>[3x]MLEANVYDNFNPNYYNISDFSMPNGKKEKRGLPIPKARCQVINYELWETGYLYTSSATLTVSVEVGDIVQILFPEVVPIEEALGKKKKLNLDMVYLVTDVDESNKATLKNYFWAMIESLDVPNAITKTTNFAIIDYLIDPNKNNLMSYGYFFNSSIFAGKATINRKAETSSAHDVAKRIFSKVQFQPTTTIQHAPSETDPRNLLFINFASRNWNRKRITTRVDIKQSVTMDTETIVERSAYNFAVVFVKNKATDDYTDPPKMYIAKNNGDVIDYSTYHGDGTDLPDVRTAKTLFYDRDDHGNPPELSTIKVEISPSTIVTRLIFNQNELLPLYVNDLVDIWYEGKLYSGYIADRVKTEFNDRLIFVESGDKPNVI;>[12x]MVRQYKIHTNLDGTDDKVWDVTNGKVRFYQPSNLGLQSTNNIWQSNGIGVMGTRSITQPQIEFKLETFGESLEENYQLMKDFVNDILSKKFVTLEYQTEIFQVYADLAL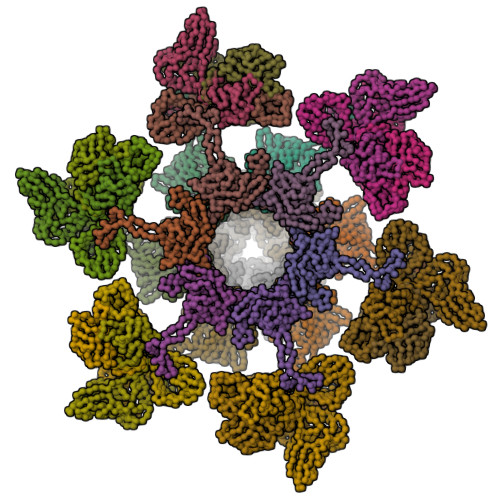ADVTKTEGYGKNGTFSEKITFDIITKWYTYENLTFDKIQNGKVIAGMSKIYGGTAPGNYKYIKGTSYTYYGESDIDRLSRWDIKEEIFSFMGILYPKLPKTPAGVRFLDDIGNEYTAIVFKTEQVQDYILINTDVNDETYQGWKGTTALNLFPVMDFERYRTRIIEKGQMELINLSKAEFKIKRKADFV;>[18x]MTIKNFTFFSPNSTEFPVGSNNDGKLYMMLTGMDYRTIRRKDWSSPLNTALNVQYTNTSIIAGGRYFELLNETVALKGDSVNYIHANIDLTQTANPVSLSAETANNSNGVDINNGSGVLKVCFDIVTTSGTGVTSTKPIVQTSTLDSISVNDMTVSGSIDVPVQTLTVEAGNGLQLQLTKKNNDLVIVRFFGSVSNIQKGWNMSGTWVDRPFRPAAVQSLVGHFAGRDTSFHIDINPNGSITWWGANIDKTPIATRGNGSYFIK>[2x]MGSMRICIFMARGLEGCGVTKFSLEQRDWFIKNGHEVTLVYAKDKSFTRTSSHDHKSFSIPVILAKEYDKALKLVNDCDILIINSVPATSVQEATINNYKKLLDNIKPSIRVVVYQHDHSVLSLRRNLGLEETVRRADVIFSHSDNGDFNKVLMKEWYPETVSLFDDIEEAPTVYNFQPPMDIVKVRSTYWKDVSEINMNINRWIGRTTTWKGFYQMFDFHEKFLK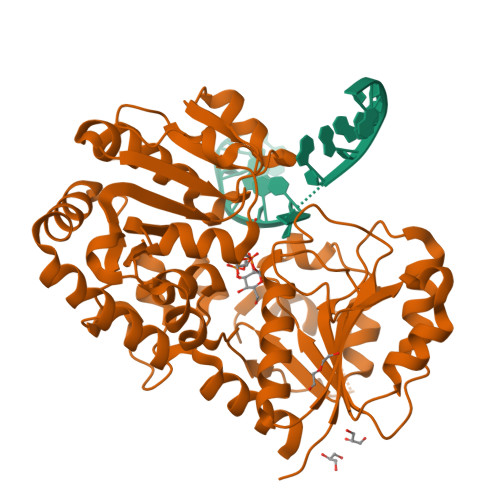PAGKSTVMEGLERSPAFIAIKEKGIPYEYYGNREIDKMNLAPNQPAQILDCYINSEMLERMSKSGFGYQLSKLNQKYLQRSLEYTHLELGACGTIPVFWKSTGENLKFRVDNTPLTSHDSGIIWFDENDMESTFERIKELSSDRALYDREREKAYEFLYQHQDSSFCFKEQFDIITK>[2x]QDWLTFQK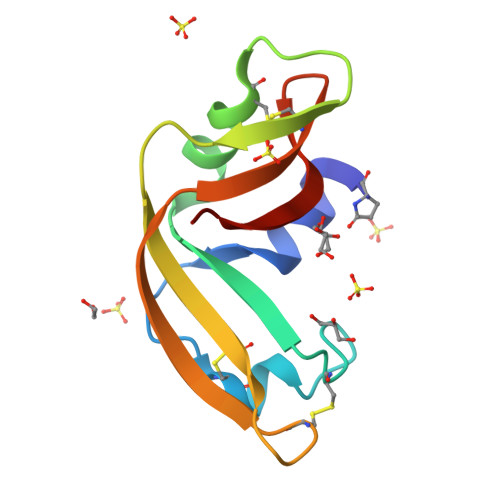KHITNTRDVDCDNIMSTNLFHCKDKNTFIYSRPEPVKAICKGIIASKNVLTTSEFYLSDCNVTSRPCKYKLKKSTNKFAVTCENQAPVHFVGVGSA> MGSSHHHHHHSSGRENLYFQGHMTDQIREHLVSML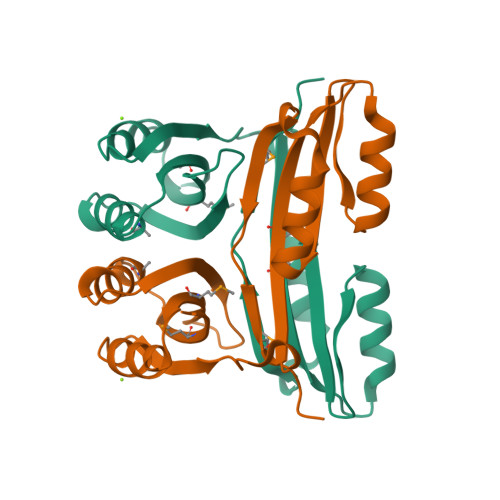VHNKPGVMRKVANLFARRGFNISSITVGESETPGLSRLVIMVKGDDKTIEQIEKQAYKLVEVVKVTPIDPLPENRVEREMALIKVRFDEDKQEIFQLVEIFRGKIIDVSREGAIIEITGARSKVEAFINLLPQKQVEEIARTGIVAMNRWNVKEGEGF>[2x]MNHKVHHHHHHMLDIGNASKTNYGVSLNEYIKLQQRNNPSNYSYSEFEKYINPAKATNKLQFLRIDKFRSVNVSGLSSRLSNKGVLTGQGQAFVNAAKAFNIDPI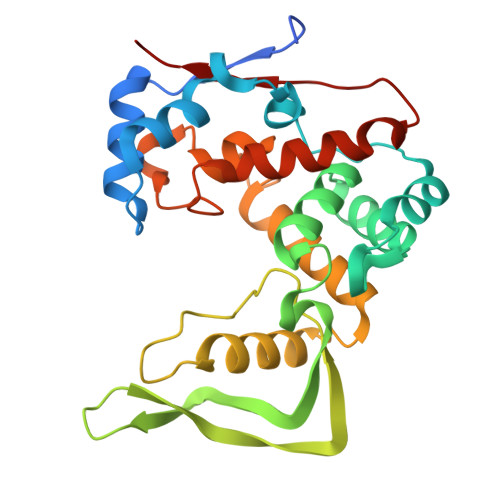YLVAQCLHETGNGTSKLAKGVTITEIADESKPIYNGNGQLVGYHMIKLSKPVTVYNLFGIGAKDNSSVFPNRALILGTTYAYNRGWTSIENAIKGAAEFVSLNYVHSSRYSQNTLYKMRYNQNVSNIWHQYATTPWYASSIADIMRSYQDLYLENNFTFDVPVFAG>MLTTKSLVERFELEMIAGEAGLNK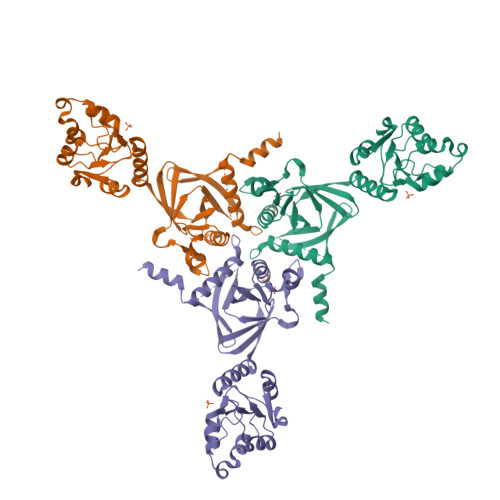QIKNTDISRPGLEMAGYFSHYASDRIQLLGTTELSFYNLLPDEERKGRMRKLCRPETPAIIVTRDLEPPEELIEAAKEHETPLITSKIATTQLMSRLTTFLEHELARTTSLHGVLVDVYGVGVLITGDSGIGKSETALELIKRGHRLVADDNVEIREISKDELIGRAPKLIEHLLEIRGLGIINVMTLFGAGSILTEKRLRLNIHLENWHKEKLYDRVGLNEETLRILDTEITKKTIPVRPGRNVAVIIEVAAMNYRLNIMGINTAEEFNDRLNAEILRNGNNGNNGEEK[2x]6-(ADENOSINE 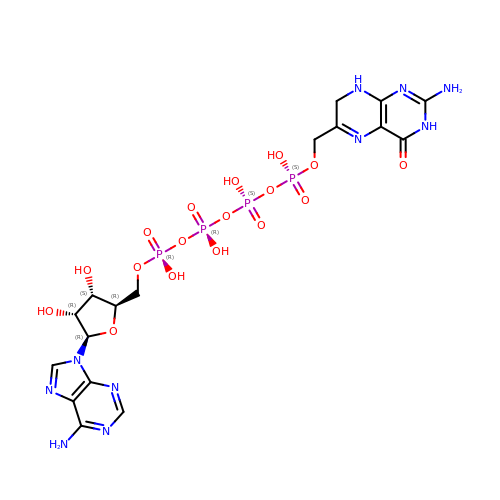TETRAPHOSPHATE-METHYL)-7,8-DIHYDROPTERIN | C17 H24 N10 O17 P4 | ZKRKFZJAQKKHKL-SUGPNEFASA-N> AMKKDSKAPCVEVFDERDGCKAAGTQKASGDDGFCV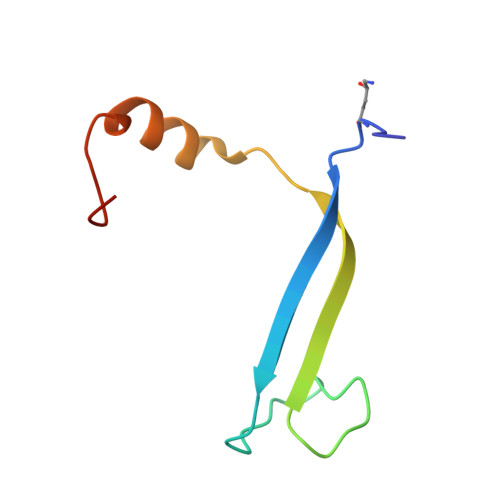KVSMKAIGFNAAEAASVTKNYGIKRFGAKSV> MSGFGGGSSGAGSLTQLLATGSMDAALTQNATRTFWKSSYQKHSLFALESINQPFTTQVQFGAESHITVNRQGDLLSWMYLKIVLPGLKVQNQADTVQPT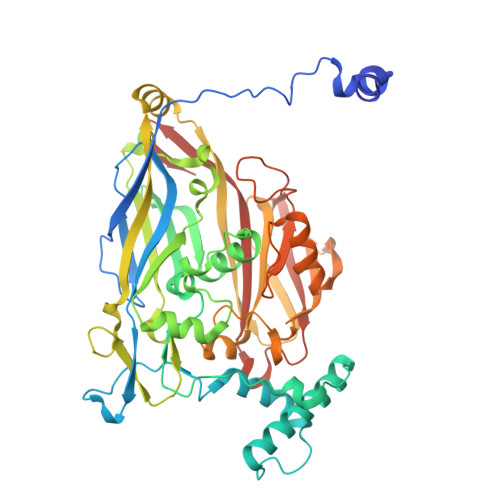QQSFASLDNDVAAQADVSHVLPYIEGAYTEASLNTKEQLIAEAKNSYEAAKYNAAPLPVAAQMQSTEMPDFDYAYWTEAIGFHLIKRAEFKVGGATIDTIWSELLFAMEELMGRAGRRLTETIGRTLRRPTELMKASRQEQILYVPLPWYFTKHPSLAFPLVAATYHNIQLWVQWAQLNSCIIKSRSNLVVLHAERNVPISDDHLRASLECTYVHLEAAERDALTANAGTQLIVQHQAHLQQVSSNNVTARLNFNFPVLEFYYFLRRKANKDAGDHFNFSGIGGRDPVVSAELLFNNTARVTQKPAVWWRAVQALQFHSSAPLTNIYSYSFSLSPEDPITPSGSANFSRLDSVELALTLQDDFGAAHDANSELFVFARSYNILKFTNGLAGLLYSN> MEAVVISGRKLAQQIKQEVRQEVEEWVASGNKRPHLSVILVGENPASHSYVLNKTRAAAVV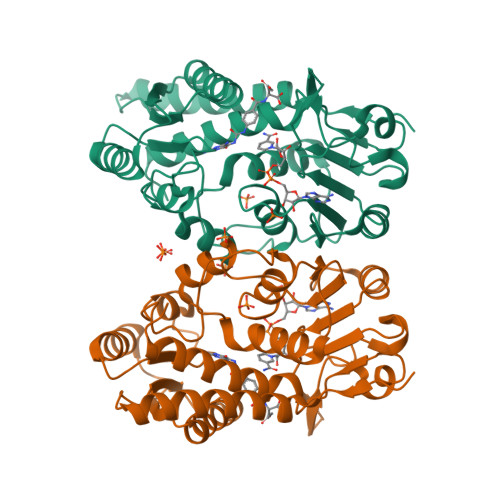GINSETIMKPASISEEELLNLINKLNNDDNVDGLLVQLPLPEHIDERRICNAVSPDKDVDGFHVINVGRMCLDQYSMLPATPWGVWEIIKRTGIPTLGKNVVVAGRSKNVGMPIAMLLHTDGAHERPGGDATVTISHRYTPKEQLKKHTILADIVISAAGIPNLITADMIKEGAAVIDVGINRVHDPVTAKPKLVGDVDFEGVRQKAGYITPVPGGVGPMTVAMLMKNTIIAAKKVLRLEEREVLKSKELGVATN>[2x]SGTATYSGNPFVGVTPWANAYYASEVSSLAIPSLTGAMATAAAAVAKVPSFMWLDTLDKTPLMEQTLADIRTANKNGGNYAGQFVVFDLPDRDCAALASNGEYSIADGGVAKYKNYIDTIRQIVVEYSDIRTLLVIEPDSLANLVTNLGTPKC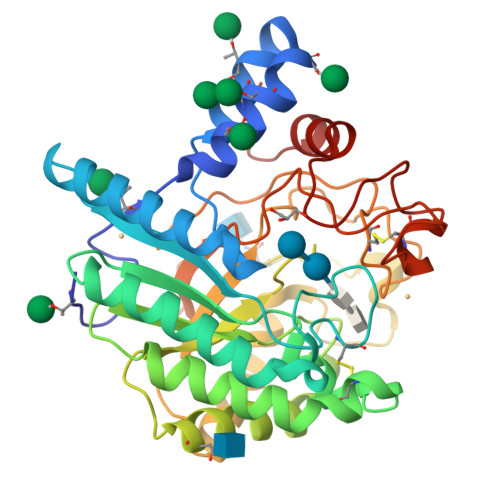ANAQSAYLECINYAVTQLNLPNVAMYLDAGHAGWLGWPANQDPAAQLFANVYKNASSPRALRGLATNVANYNGWNITSPPSYTQGNAVYNEKLYIHAIGPLLANHGWSNAFFITDQGRSGKQPTGQQQWGDWCNVIGTGFGIRPSANTGDSLLDSFVWVKPGGECDGTSDSSAPRFDSHCALPDALQPAPQAGAWFQAYFVQLLTNANPSFL pentane-1,3,5-tricarboxylic acid | C8 H12 O6 | 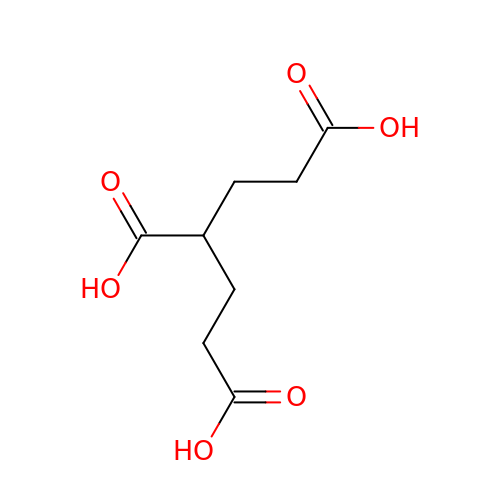ROTJZTYLACIJIG-UHFFFAOYSA-N>MNYFVGNSLGVNLTGIEKAIINRLNLFKEMGRPAQCVFLSWNRYLYRNAQNYITSSDYINMYDFFQEATYLERNEPFDWLSYWTDECHYTLKHVENSHDFRIYDQERFLMYAHFQDPKYRILDYVNHFDSQRRKVKRDFYDVRGFLSCSRILVDKQQTLCEFFYNPEGDTKLEKYFSYKDGKPEVQKIIVYYANKQYFFNNETELGAFFIKQLYQHGDLFFSDRNVYTAPIFNLTPESIPVVAVLHSTHIKNIDALDSSPFKNVYKAMFENLSRYRAIIVSTEQQKLDVEKRINHTIPVVNIPVGYSETIDTPVQTL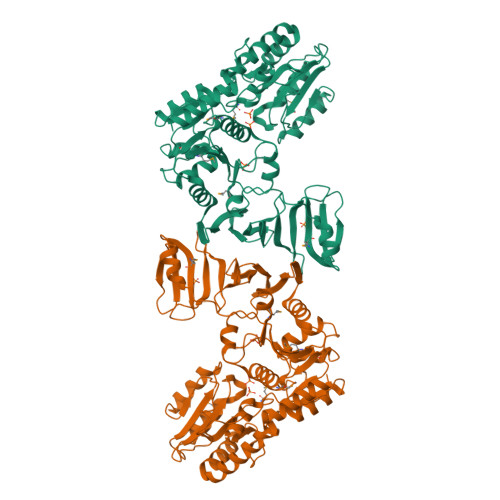DQRSVKLISVARYSPEKQLHQQIELIKRLVSYVPKIELHMYGFGSESKKLNELIQKYGLENHVYLRGFLSNLDQEYSDAYLSLITSNMEGFSLALLESLAHGVPVISYDIKYGPNELITSDFNGYLITKNDEDALFDKVKYVIDHPEVQQRLSKGSLAKAQQYSKASLIKQWDQFVRLILEHHHHHH[2x]> MDRNIIMTETPIRIATRQSPLALWQANYVKDALMAAHPGLQVELVTMVTRGDVILDTPLAKVGGKGLFVKELEIAMLEGRADLAVHSMKDVPVDF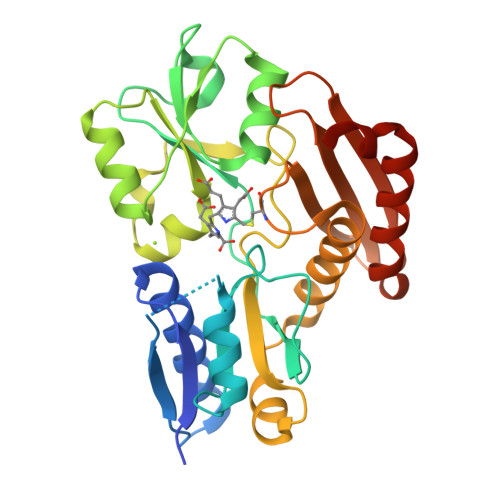PDGLGLVTICEREDPRDAFVSNTYAKIEDLPSGAIVGTCSLRRQCQLKAARPDLVIKELRGNVGTRLSKLDAGEYDAIILAAAGLKRLELESRIRSFIEPEQSLPAVGQGAVGIECRVNDQRVRALLAPLNHADTADRVRCERAMNLTLQGGCQVPIGSYALLEGDTIWLRALVGEPDGSQIVRGEIRGPRTQAEQLGITLAEQLLSQGAKEILERLYCDHE> MNDQTQFTERALTILTLAQKLASDHQHPQLQPIHILAAFIETPEDGSVPYLQNLIEKGRYDYDLFKKVVNRNLVRIPQQQPAPAEITPSYALGKVLQDAAKIQKQQKDSFIAQDHILFALFNDSSIQQIFKEAQVDIEAIKQQALELRGNTRIDSRGADTNTPLEYLSKYAIDMTEQARQGKLDPVIGREEEIRSTIRVLARRIKSNPCLIGEPGIGKTAIIEGVAQRIIDDDVPTILQGAKLFSLDLAALTAGAKYKGDFEERFKGVLKEIEESKTLIVLFIDEIHMLMGNGKDDAANILKPALSRGQLKVIGATTNNEYRSIVEKDGAFERRFQKIEVAEPSVRQTVAILRGLQPKYEIHHGVRILDSALVTAAQLAKRYLPYRRLPDSALDLVDISCAGVAVARDSKPEELDSKERQLQLIQVEIKALERDEDADSTTKDRLKLARQKEASLQEELEPLRQRYNEEKHGHEELTQAKKKLDELENKALDAERRYDTATAADLRYFAIPDIKKQIEKLEDQVAEEERRAGANSMIQNVVDSDTISETAARLTGIPVKKLSESENEKLIHMERDLSSEVVGQMDAIKAVSNAVRLSRSGLANPRQPASFLFLGLSGSGKTELAKKVAGFLFNDEDMMIRVDCSELSEKYAVSKLLGTTAGYVGYDEGGFLTNQLQYKPYSVLLFDEVEKAHPDVLTVMLQMLDDGRITSGQGKTIDCSNCIVIMTSNLGAEFINSQQGSKIQESTKNLVMGAVRQHFRPEFLNRISSIVIFNKLSRKAIHKIVDIR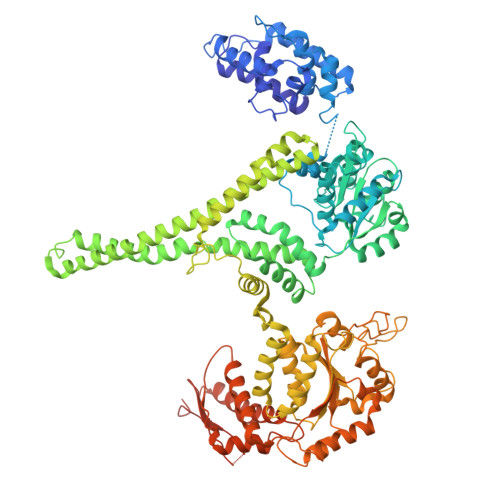LKEIEERFEQNDKHYKLNLTQEAKDFLAKYGYSDDMGARPLNRLIQNEILNKLALRILKNEIKDKETVNVVLKKGKSRDENVPEEAEECLEVLPNHEATIGADTLGDDDNEDSMEIDDDLD>[3x]HHHHHQSEFIKDSKASIELRNFYFNRDFRQEGASQSKAEEWAQGFLLRYESGYTEGTIGFGVDAIGLLGVKLDSSPDRSGTGLLKRDRETGRAQDDYGEAGITAKLRASKSTLKIGTLTPKLPVIMPNDSRLLPQTFQGGALNSMEIDGLTLDAGRLKKVNQRDSSDNEDMTITGGGKRQIVVRSGLTSDKFDFAGGSYKWTDNLSTSYHYGKLDNFYKQHYLGLVHTLPIADKQSLKSDIRWARSTDDGSSNVDNKALNAMFTYSLGYHAFGVGYQKMSGDTGFAYINGADPYLVNFIQIGDFANKDEKSWQARYDYNFAGVGIPGLTFMTRYVKGDNIDLLTTSGEGKEWERDMDIAYVFQSGPLKNLGVKWRNATMRTNYTNDYDENRLIVSYTLPLW

In such microorganisms, the majority of small molecules are taken up by members of the OprD outer membrane protein family. Here we show that OprD channels require a carboxyl group in the substrate for efficient transport, and based on this we have renamed the family Occ, for outer membrane carboxylate channels. As expected from pairwise sequence identities that range from 35%–50%, the Occ proteins share a similar architecture, with a slightly off-center constriction formed by the inward-folded extracellular loops L3 and L7 and residues in the barrel wall. The transport data demonstrate that Occ channels have a pronounced preference for substrates with a carboxyl group, due to the universal presence of a basic ladder on one side of the barrel wall.

To determine if the phylogenetic subdivision of Occ proteins exists at the structural level, we determined X-ray crystal structures for seven Occ family members (OccD2, OccD3, and OccK2–K6). A comparison of the crystal structures suggests that the division into the OccD and OccK subfamilies occurs on a structural level as well; the OccD subfamily members of which structures were determined have much smaller pores than those of the OccK subfamily. The pores of the proteins within the OccK subfamily show a considerable variation in size and shape, suggesting differences in substrate preferences within subfamilies as well. For OccK channels, conductance values are on average somewhat larger than those of OccD subfamily members, ranging from ∼50 pS for OccK4 to ∼300 pS for OccK1, OccK5, and OccK7. These data are consistent with the fairly large pores observed in the six crystal structures of members of this subfamily. OccK channels, on the other hand, appear to be less selective and facilitate passage of a wider variety of substances, with a preference for cyclic compounds.>AQESPAFIDPASWNTPFNGIAQVACHNCYEKQYANTFSSVLDSVRTLELDFWDQRDAVSGGSPHHWFVRHNPGTLFQSGNDNNCTGDGTGKNDLEACLNDVKNWSDKHPGHFPITLILDKKQGWSKESSGRTPKDFDELVARVFQGKLFTPQDLATHIGSGAGALQGNLKGKSWPTANDL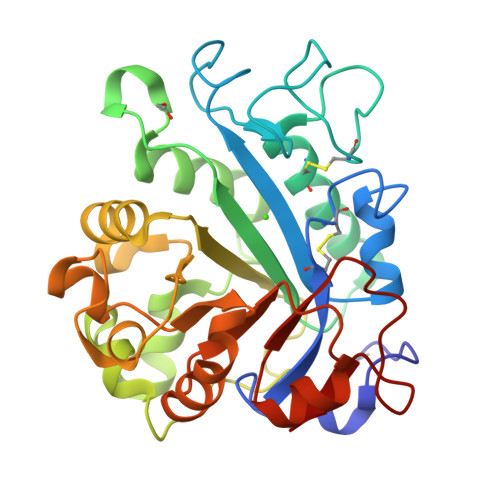QGKVLLVLNHSENQKLSQYAEARTSKAKVFISPVTNGQNDISGKVSGMSSQSSGYVAMNNMGKGDKSWAKQAFAYSHIGRVWGDDEVSFAQHINQKINLSAYYRFAAQSAGGYRIRPF[2x]> MKDSGDSKDQQLMVALRVRPISVAELEEGATLIAHKMDEQMVVLMDPMEDPDDILRAHRSREKSYLFDVAFDFTATQEMVYQATTKSLIEGVISGYNATVFAYGPTGCGKTYTMLGTDHEPGIYVRTLNDLFRAIEETSNDMEYEVSMSYLEIYNEMIRDLLNPALGYLELREDSKGVIQVAGITEVSTINAKEIMQLLMKGNRQRTQEPTAANQTSSRSHAVLQVAVRQRSRVKNILQEVRQGRLFMIDLAGSERASQ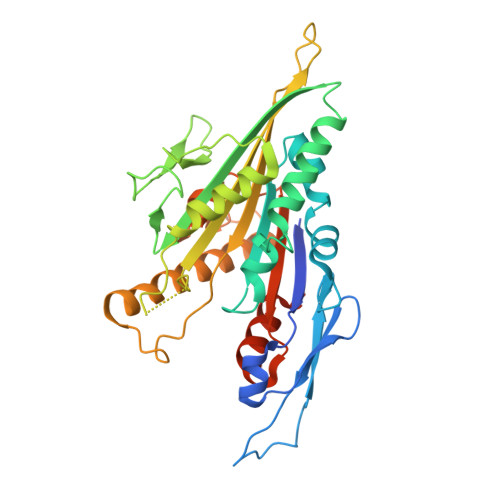TQNRGQRMKEGAHINRSLLALGNCINALSDKGSNKYINYRDSKLTRLLKDSLGGNSRTVMIAHISPASTAFEESRNTLTYAGRAKNIRTRVKQNHHHHHHH>[2x]MGSPDIELVYKNRGFYKHYGVRFGGHIYHLNSQDILSTAITGKSDFIKEEDDGKWVHAMTAPLDYFTEKYINSMVGSKHIFSATSNCETIARDLFPGRKEITQSKALGIIGVILLSASLLSLLAVPWDYSSLQTVYNQLEHHHHHH

Parechoviruses, including *Parechovirus A* that infects humans as well as *Parechovirus B* (formerly Ljungan virus) and *Parechovirus C* (formerly Sebokele virus) that infect rodents, belong to a group of picornaviruses whose 2A proteins, instead of being proteases, contain a conserved H-box and NC-motif and are homologous to a small cellular lipid-modifying enzyme (PLAAT3) that acts as a host factor, enabling the picornavirus life cycle. Despite the common evolutionary origin, 2A^H/NC^ proteins and PLAAT3 have no conserved function, as the active site of the viral proteins cannot support catalysis. Our structural analysis has shown that the topological rearrangement first observed in HPeV1 and leading to the apparent destruction of the active site configuration of the enzyme is indeed a general feature of *Parechovirus* 2A proteins. The C-terminal α5 region, which is a unique C-terminal extension so far only observed in *Parechovirus* 2A proteins, clearly plays a central role in determining the order of oligomerization as well as other correlated and sometimes far-reaching structural rearrangements.

To see whether this destroyed active site is also preserved in other species of the genus *Parechovirus*, we decided to expand our structural characterization to members of the *Parechovirus B* species. We determined the structure of LV1-2A_2_ to 1.73 Å resolution in P2_1_2_1_2_1_ with two molecules in the asymmetric unit and refined it to 21.45% Rfree, a Molprobity score of 1.25 (98^th^ percentile) without any Ramachandran outliers and a Ramachandran Z score of 0.06 ±0.61. The final model included 103 water molecules, however, due to missing electron density, the C-terminal residues 130-135 in chain A and residues 123-135 in chain B as well as the C-terminal hexahistidine-tag could not be modeled. In *Parechovirus B* 2A_2_, the stretch of amino acids corresponding to the C-terminal α5 helix in *Parechovirus A* and *C* 2A proteins, is either at least partially disordered (LV1-2A_2_) or had been truncated to obtain diffraction quality crystals (LV4-2A_2_). Taking a closer look at monomer A of LV1-2A_2_, in which only the last six residues are disordered, we can see that α4 extends for an extra four residues, the same as in SEBV1-2A_2_. However, whereas the remaining C-terminal stretch encompassing α5 in SEBV1-2A_2_ folds back on top of α4 and nestles against α2, in LV1-2A_2_, this stretch falls more to the side of α4 and towards the back of the β-sheet. There, it appears to be anchored by hydrogen bonds formed between main chain carbonyls of the C-terminal stretch with the side chains of Asn9 (β1), Lys14 (β2), and the last ordered residue H-bonds to the side chain hydroxyl of Tyr62 (α2). In conjunction with this different C-terminal organization we also see a different packing of the two monomers forming the dimer, though the majority of the interface contacts are still formed by the α-helices ([Fig fig2]).> MTVRKNQATLTADEKRRFVAAVLELKRSGRYDEFVRTHNEFIMSDTDSGERTGHRSPSFLPWHRRFLLDFEQALQSVDSSVTLPYWDWSADRTVRASLWAPDFLGGTGRSTDGRVMDGPFAASTGNWPINVRVDSRTYLRRSLGGSVAELPTRAEVESVLAISAYDLPPYNSASEGFRNHLEGWRGVNLHNRVHVWVGGQMATGVSPNDPVFWLHHAYVDKLWAEWQRRHPDSAYVPTGGTPDVVDLNETM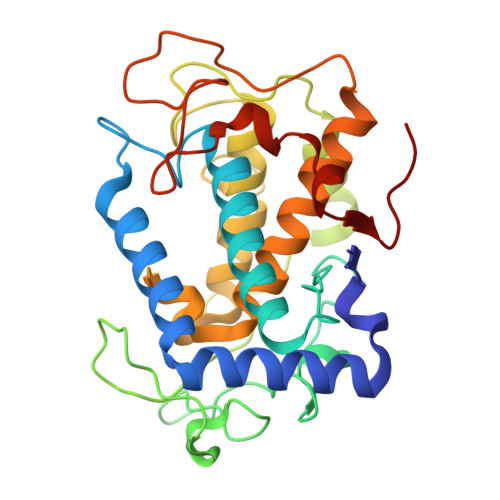KPWNTVRPADLLDHTAYYTFDALEHHHHHH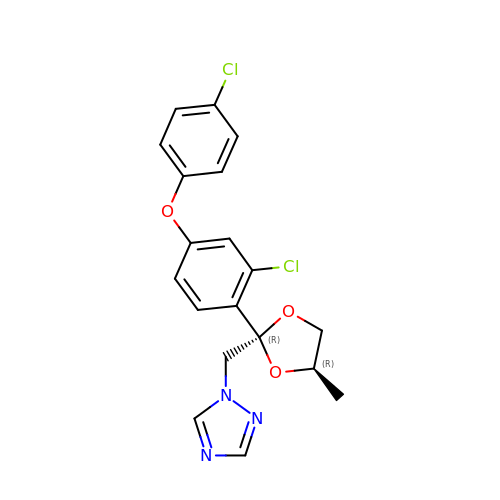1-[[(2~{R},4~{R})-2-[2-chloranyl-4-(4-chloranylphenoxy)phenyl]-4-methyl-1,3-dioxolan-2-yl]methyl]-1,2,4-triazole | C19 H17 Cl2 N3 O3 | BQYJATMQXGBDHF-YJYMSZOUSA-N>[2x]EPEWTYPRLSCQGSTFQKALLISPHRFGEARGNSAPLIIREPFIACGPKECKHFALTHYAAQPGGYYNGTREDRNKLRHLISVKLGKIPTVENSIFHMAAWSGSACHDGREWTYIGVDGPDSNALIKIKYGEAYTDTYHSYANNILRTQESACNCIGGDCYLMITDGS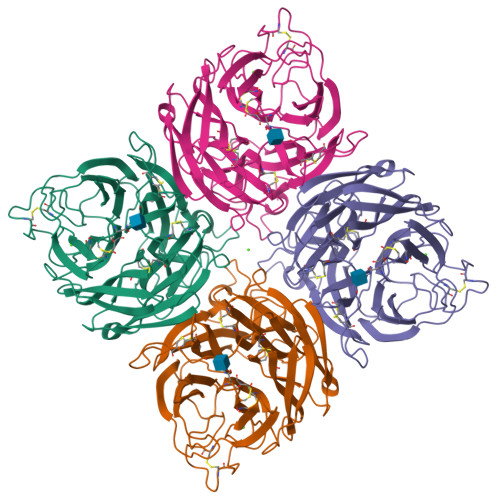ASGISKCRFLKIREGRIIKEIFPTGRVEHTEECTCGFASNKTIECACRDNSYTAKRPFVKLNVETDTAEIRLMCTETYLDTPRPDDGSITGPCESNGDKGRGGIKGGFVHQRMASKIGRWYSRTMSKTERMGMELYVRYDGDPWTDSDALAHSGVMVSMKEPGWYSFGFEIKDKKCDVPCIGIEMVHDGGKKTWHSAATAIYCLMGSGQLLWDTVTGVDMAL>MAHHHHHHRKKTKEQIAHLKASFLQSQFPDDAEVYRLIEVTGLARSEIKKWFSDHRYRCQRGIVHI[2x]

Zhx1 to 3 (zinc-fingers and homeoboxes) form a set of paralogous genes encoding multi-domain proteins. ZHXs are multidomain proteins comprising two C2H2 zinc finger motifs and five homeodomains. In transient co-transfection assays ZHX isoforms have all been shown to function as transcriptional repressors. Whilst many 3-D structures of homeodomains have been determined by crystallography and NMR, we report two ZHX homeodomain structures which contain novel features.

The structure determination of crystals grown using protein derived from OPPF_2273 (ZHX2 HD2-3) revealed a number of unexpected features. Firstly, it became clear during the refinement that the two ZHX2 homeodomains present within the asymmetric unit were of identical amino acid sequence and were not covalently linked, unexpected for protein derived from the bidomain HD2-HD3 construct. The sequence of the observed domain corresponded to that of HD2 indicating cleavage of HD2-HD3 had occurred and that HD2 preferentially crystallized compared to HD3. The second unexpected feature for ZHX2 HD2 homeodomain was the unusual conformation and dimer formation. The change involved the rotation of helix I by ~180° compared to the usual homeodomain conformation, giving a more opened out structure with some disruption of the hydrophobic core. A ZHX2 HD2 homodimer is observed in the crystal which is further stabilized by a disulfide bridge formed by linkage of Cys494s. The switching of the positions of the two helices I in ZHX2 HD2 provides an example of 'domain swapping'. Thus, this homeodomain conformation appears to be unique amongst reported crystal/NMR structures for this domain class. However, the dimer we observe in the crystal structure serves to bury some of the exposed hydrophobic residues at the interface between the subunits. In contrast, for ZHX2 HD2 the rearranged conformation involving movement of helix I, relative to the canonical homeodomain fold, would disrupt the normal DNA binding site, however, protein-protein interact is possible as a homodimer is observed.> MEMPQLSKWNQDSRNDAMENTLLVSHVLPNISVAQIHNALDGISFVQHFSLSTINLIKNDERSLWVHFKAGTNMDGAKEAVDGIQLDSNFTIESENPKIPTHTHPIPIFEIASSEQTCKNLLEKLIRFIDRASTKYSLPNDAAQRIEDRLKTHASMKDDDDKPTNFHDIRLSDLYAEYLRQVATFDFWTSKEYESL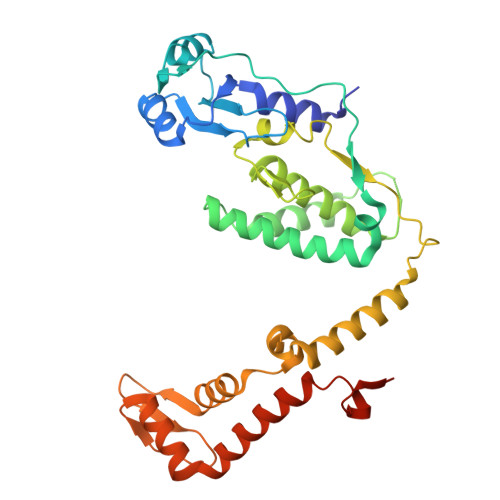IALLQDSPAGYSRKKFNPSKEVGQEENIWLSDLENNFACLLEPENVDIKAKGALPVEDFINNELDSVIMKEDEQKYRCHVGTCAKLFLGPEFVRKHINKKHKDWLDHIKKVAICLYGYVLDPCRAMDPKVVSSAWSHPQFEK>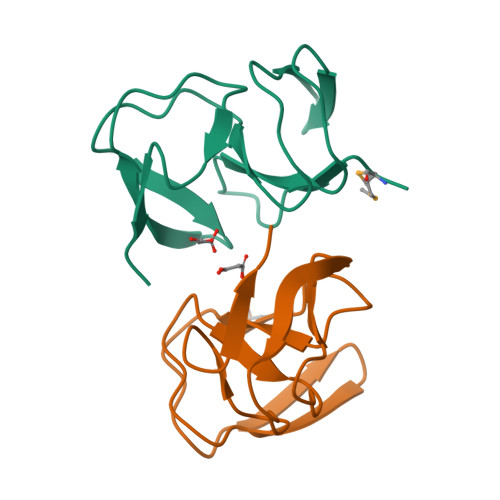[8x]MGSSHHHHHHSSGRENLYFQGMQYIKIHALDNVAVALADLAEGTEVSVDNQTVTLRQDVARGHKFALTDIAKGANVIKYGLPIGYALADIAAGEHVHAHNTRTNL> MH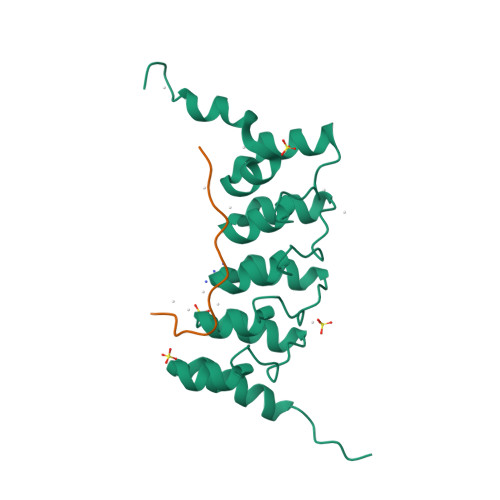HHHHHSSGRENLYFQGSTTPLLANSLSVHQLAAQGEMLYLATRIEQENVINHTDEEGFTPLMWAAAHGQIAVVEFLLQNGADPQLLGKGRESALSLACSKGYTDIVKMLLDCGVDVNEYDWNGGTPLLYAVHGNHVKCVKMLLESGADPTIETDSGYNSMDLAVALGYRSVQQVIESHLLKLLQNIKE;> KAFVHMPTLPNLDFHKT>[3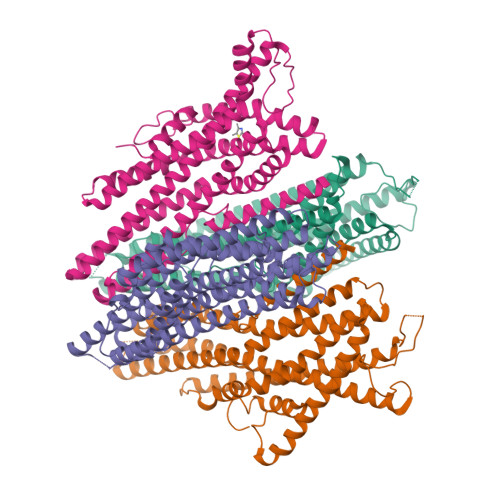x]MKFKHQGLVADLLPNIRVMQGVGHFMFNYYSEGKKFPHRIYCIVTLLLLLLQYGMMAVNLMMESDDVDDLTANTITMLFFLHPIVKMIYFPVRSKIFYKTLAIWNNPNSHPLFAESNARFHALAITKMRRLLFCVAGATIFSVISWTGITFIEDSVKRITDPETNETTIIPIPRLMIRTFYPFNAMSGAGHVFALIYQFYYLVISMAVSNSLDVLFCSWLLFACEQLQHLKAIMKPLMELSATLDTVVPNSGELFKAGSADHLRESQGVQPSGNGDNVLDVDLRGIYSNRQDFTATFRPTAGTTFNGGVGPNGLTKKQEMLVRSAIKYWVERHKHVVRLVTAVGDAYGVALLLHMLTTTITLTLLAYQATKVNGVNVYAATVIGYLLYTLGQVFLFCIFGNRLIEESSSVMEAAYSCHWYDGSEEAKTFVQIVCQQCQKAMSISGAKFFTVSLDLFASVLGAVVTYFMVLVQLK;> MARLVLHEVRYVLMAMLYISRGMAKQIQNSTIDLYVYWFLTFIPIASLCVPQFTYLVVDTKSLIDFISVLVPITEILLTNGKMIICNVKRGKIINLINQVQVAWDECAKSEHLEIQTLITATAKKTKIFVIIYTTSFLLICVEYSSMPLFKLIYHSAVYGKQSNYTIALPYLSRFAYSTESTTSFAWTYFFILLGVYLLALTLSGFDSLFATLVMHVKMMFKVLKFEIEQLGLDLSAGKSHVELQAKLKQIILKHKTNLSLIEQLEDGFSFFLMAQFLTSSILVCVVLYELTMVFGWNEDTFKTVTYLPGAILQLFLFCWYAQQITEEARLVSDHIYNIPWYLADPKLQKDILTFMVKAQKPTGVTASKFYMVTLQTFQRISSTSYSYFTLLQTINQQ> SLTFYPAWLTVSEGANATFTCSLSNWSEDLMLNWNRLSPSNQTEKQAAFSNGLSQPVQDARFQIIQLPNRHDFHMNILDTRRNDSGIYLCGAISLHPKLKIEESPGAELVVTERILE;> MLFTVTAPKEVYTVDVGSSVSLECDFDRRECTELEGIRASLQKVENDTSLQSERATLLEEQLPLGKA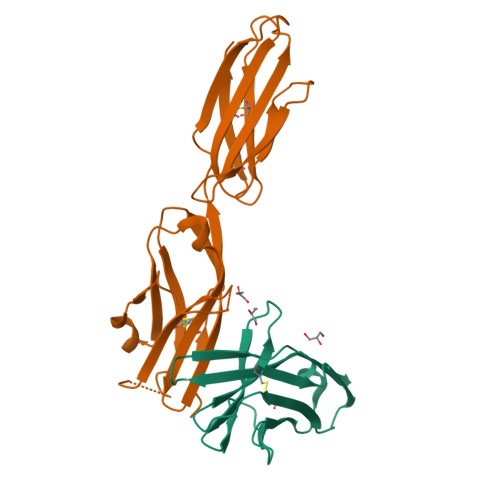LFHIPSVQVRDSGQYRCLVICGAAWDYKYLTVKVKASYMRIDTRILEVPGTGEVQLTCQARGYPLAEVSWQNVSVPANTSHIRTPEGLYQVTSVLRLKPQPSRNFSCMFWNAHMKELTSAIIDPLSRMEPKVPRT>SSIIRKVISTSKAPAAIGAYSQAVLVDRTIYVSGQIGMDPSSGQL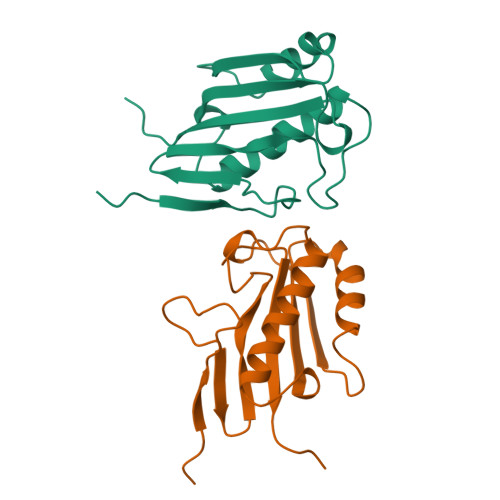VPGGVAEEAKQALKNLGEILKAAGCDFTNVVKTTVLLADINDFGTVNEIYKTYFQGNLPARAAYQVAALPKGSRIEIEAIAVQGPFTTAGL[2x]>[2x]GSHMARYDSLLQALGNTPLVGLQRLSPRWDDGRDGPHVRLWAKLEDRNPTGSIKDRPAVRMIEQAEADGLLRPGATILEPTSGNTGISLAMAARLKGYRLICVMPENTSVERRQLLELYGAQ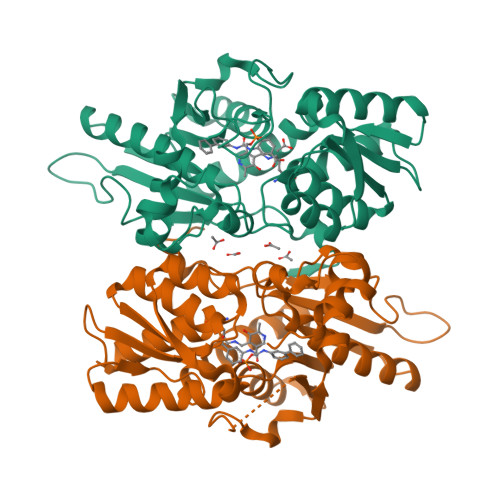IIFSAAEGGSNTAVATAKELAATNPSWVMLYQYGNPANTDSHYCGTGPELLADLPEITHFVAGLGTTGTLMGTGRFLREHVANVKIVAAEPRYGEGVYALRNMDEGFVPELYDPEILTARYSVGAVDAVRRTRELVHTEGIFAGISTGAVLHAALGVGAGALAAGERADIALVVADAGWKYLSTGAYAGSLDDAETALEGQLWA BET proteins are chromatin-associated factors that regulate transcription and chromatin remodelling. BET proteins bind chromatin through their two BDs (BD1 and BD2), which specifically recognize histones acetylated on lysine residues. The BDs from C. albicans Bdf1 (CaBdf1) share 31–46% sequence identity with human BET BDs and 58–66% identity with those from ScBdf1 and hence are likely to bind multi-acetylated H3 and H4 tails. In conclusion, Bdf1 BDs are required for the viability and virulence of C. albicans and can be selectively targeted by small-molecule inhibitors without compromising human BET BD function.

To identify features differentiating the ligand-binding pockets of human and fungal BET BDs, we determined crystal structures for CaBdf1 BD1 and BD2. These structures exhibit the canonical BD fold (comprising helices Z,A,B and C, with the ZA and BC loops defining the ligand-binding pocket) and closely resemble those of their human BET counterparts (mean pairwise root-mean-square deviations (RMSDs) ≤1.5 Å; Supplementary Table 3). The ligand-binding loops are structurally well conserved, including nearly all water molecules implicated in ligand recognition, although the overall binding surfaces are less negatively charged in CaBdf1. Superimposing the CaBdf1 BD structures onto that of JQ1-bound Brd4 BD1 reveals no major steric clashes between JQ1 and the fungal BDs. However, whereas JQ1 fits snugly into the Brd4-binding pocket, the fit with the CaBdf1-binding pockets is poor. Replacement of Brd4 residue Leu94 by a Val or Ile residue further contributes to the poor fit. In addition, the p-chlorophenyl group of JQ1 occupies a groove in Brd4, which is absent (BD1) or shallower (BD2) in CaBdf1 (asterisks in Fig. 4c). More generally, recognition of the four BETi compounds by human BET BDs involves 16 residues, including the eight signature residues previously used to classify human BD-binding sites. Five of these residues in BD1 and four in BD2 are invariant across human BET proteins but diverge in CaBdf1 (magenta arrows in Fig. 5), including the WPF-shelf Trp residue and the Leu residue opposite this shelf, at signature positions 1 and 3, respectively. Remarkably, nearly all of these residues have shorter side chains in CaBdf1 than in the human BET proteins, implying that selective CaBdf1 inhibition could conceivably be achieved via small molecules that clash sterically with the human, but not fungal, side chains. Nevertheless, an inhibitor that targets both CaBdf1 BDs without inhibiting human BET BDs is in principle achievable, because the WPF-shelf Trp residue at signature position 3 in human BET BDs is bulkier than the corresponding (Val and Phe) residues in both CaBdf1 BD1 and BD2.

> AMGAAELRFCNQTIKELMSKKHYNYNFPFLAPVDTVALNIPNYNEIVKQPMDLGTIQSKLANNEYENADDFEKDVRLVFKNCYLFNPEGTDVNMMGHRLEAVFDKKWAN> MAPDMKLFAGNATPELAQRIANRLYTSLGDAAVGRFSDGEVSVQINENVRGGDIFIIQSTCAPTNDNLMELVVMVDALRRASAGRITAVIPYFGYARQDRRVRSARVPITAKVVADFLSSVGVDRVLTVDLHAEQIQGFFDVPVDNVFGSPILLEDMLQLNLDNPIVVSPDIGGVVRARAIAKLLNDTDMAIIDKRRPRANVSQVM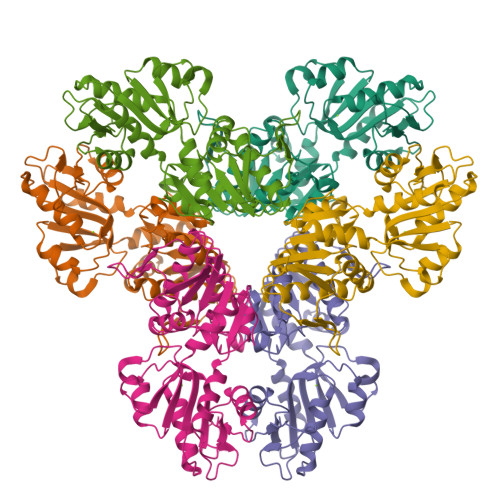HIIGDVAGRDCVLVDDMIDTGGTLCKAAEALKERGAKRVFAYATHPIFSGNAANNLRNSVIDEVVVCDTIPLSDEIKSLPNVRTLTLSGMLAEAIRRISNEESISAMFEH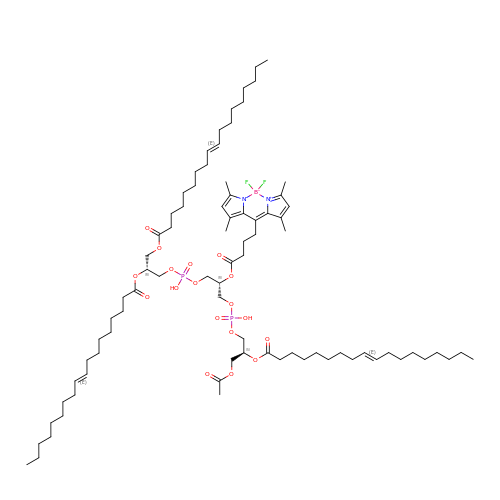[(2R,5R,11R,14S,24E)-14-[(acetyloxy)methyl]-8-{[5-(3,5-dimethyl-1H-pyrrol-2-yl-kappaN)-5-(3,5-dimethyl-2H-pyrrol-2-ylidene-kappaN)pentanoyl]oxy}-5,11-dihydroxy-2-{[(9E)-octadec-9-enoyl]oxy}-5,11,16-trioxo-4,6,10,12,15-pentaoxa-5lambda~5~,11lambda~5~-diphosphatritriacont-24-en-1-yl (9E)-octadec-9-enoatato](difluoro)boron | C82 H139 B F2 N2 O18 P2 | GDYLGRNGCDWDQL-UUEIIFSHSA-N6-[4-(3-chloro-4-fluorophenyl)-1-(2-hydroxyethyl)-1H-imidazol-5-yl]imidazo[1,2-b]pyridazine-3-carbonitrile 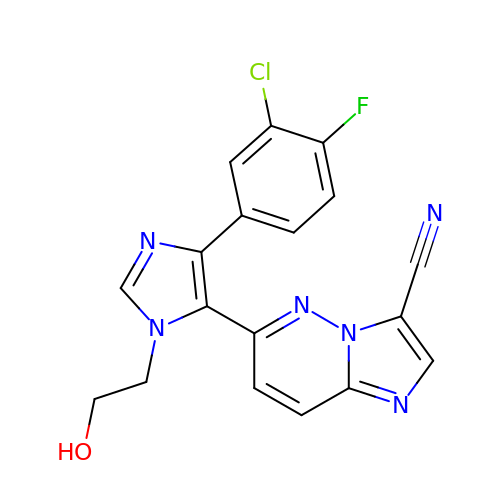| C18 H12 Cl F N6 O | VZZBCNXVZFAIQX-UHFFFAOYSA-N>MAHHHHHHVGTFENITAAPADPILGLADLFRADERPGKINLGIGVYFDETGKIPVLTSVKKAEQYLLENETTKTYLGIDGIPEFGRCTQELLFGKGSALINDKRARTAQTPGGTGALRVAADFLAKNTSVKRVWVSNPSWPNHKSVFNSAGLEVREYAYYDAENHTLDFDALINSLNEAQAGDVVLFHGCCHNPTGIDPTLEQWQTLAQLSVEKGWLPLFDFAYQGFARGLEEDAEGLRAFAAMHKELIVASSYSKNFGLYNERVGACTLVAADSETVDRAFSQMKAAIRANYSNPPAHGASVVATILSNDALRAIWEQELTDMRQRIQRMRQLFVNTLQEKGANRDFSFIIKQNGMFSFSGLTKEQVLRLREEFGVYAVASGRVNVAGMTPDNMAPLCEAIVAVL[2x]

E. coli aspartate aminotransferase (AAT) is a pyridoxal phosphate (PLP)-dependent enzyme that catalyses the reversible transamination of l-aspartate with α-ketoglutarate, yielding oxaloacetate and l-glutamate. During its catalytic cycle, AAT undergoes hinge movement to switch between an open conformation, in the ligand-free form, and a closed conformation upon association with substrates or inhibitors. Using our approach, we enrich the less populated but catalytically active closed conformation in order to increase catalytic efficiency (kcat/KM) with the non-native substrate l-phenylalanine, leading to altered substrate selectivity. Steady-state kinetics reveal kcat/KM increases of up to 100-fold towards this aromatic amino acid, resulting in a selectivity switch of up to 1900-fold, and structural analyses by room-temperature X-ray crystallography and multitemperature nuclear magnetic resonance (NMR) spectroscopy confirm that the conformational landscape is remodeled to favor the target state.

For example, the VFIT mutant from the Closed Library contains Val, Phe, Ile, and Thr residues at positions 35, 37, 43, and 64, respectively. To obtain structures in the absence of maleate, we applied a rigorous crystal soaking method to serially dilute and extract the inhibitor from the crystallized enzymes. Superposition of bound and unbound structures for each variant confirmed that closed library mutants VFIT and VFIY remained in the closed conformation in the inhibitor-free form, similar to HEX, while OpenLow variant VFCS and OpenHigh variant AIFS adopted the open conformation, similar to WT. Overlay of AAT structures (Chain A) in the presence and absence of maleate show transition from open to closed states upon inhibitor binding for WT, VFCS, and AIFS, but not for HEX, VFIT, and VFIY, which already adopt the closed conformation in the absence of bound inhibitor. We next analyzed two mutants from the Closed library (VFIT and VFIY). 19F NMR spectra at 278 K for both mutants showed a narrow peak centered at approximately ‒60.2 ppm that is similar to that of WT. Spectra of these variants also showed another broad peak centered at approximately ‒61.2 ppm that is similar to the HEX peak characteristic of the closed conformation. The relative intensity of the two peaks showed similar temperature dependence, with an increase in the relative intensity of the WT-like peak as temperature was increased to 308 K. Peak deconvolution and integration were used to evaluate the population of the two states, and confirmed that at low temperatures both VFIT and VFIY favor the state resembling that adopted by the closed HEX mutant (T < 288 K or 283 K, respectively). However, unlike HEX, at higher temperatures the alternate conformation with the WT-like peak becomes the favored state.> MKAMILAAGKGERMRPLTLHTPKPLVPVAGQPLIEYHLRALAAAGVTEVVINHAWLGQQIEDHLGDGSRFGLSIRYSPEGEPLETGGGIFKALPLLGDAPFLLVNGDVWTDYDFARLQAPLQGLA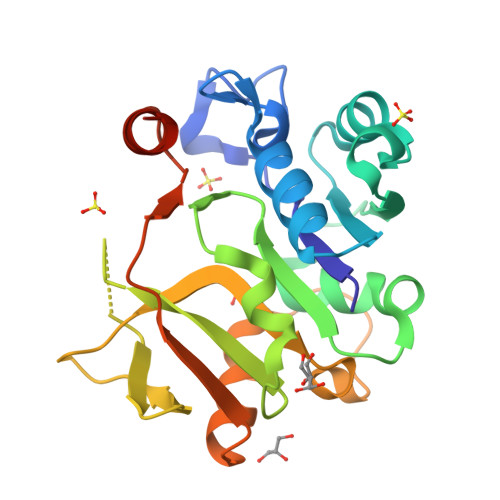HLVLVDNPGHHGRGDFRLVGEQVVDGDDAPGTLTFSGISVLHPALFEGCQAGAFKLAPLLRQAMAAGKVSGEHYRGHWVDVGTLERLAEAESLIGERALEHHHHHH> MAHHHHHHVDDDDKMVSTTPAAGVLD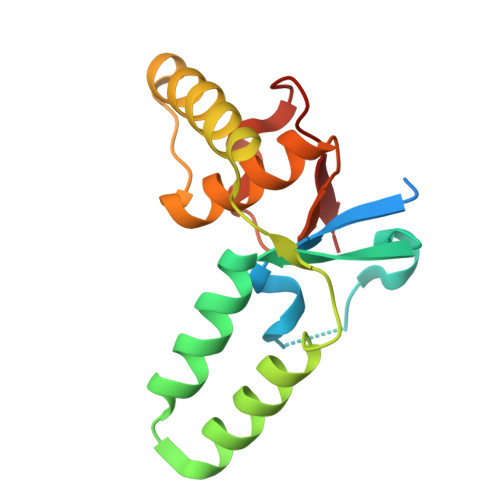TSVFIATESGRQLDEALIPDRVATTVVTLAELRVGVLAAATTDIRAQRLATLESVADMETLPVDDDAARMWARLRIHLAESGRRVRINDLWIAAVAASRALPVITQDDDFAALDGAASVEIIRV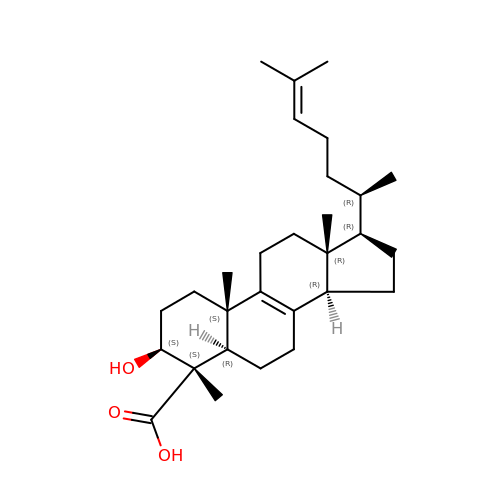(3beta,4alpha,5beta,14beta)-3-hydroxy-4-methylcholesta-8,24-diene-4-carboxylic acid | C29 H46 O3 | MYWAIWDQTCHPTH-LJAIZBFVSA-N>MTMITHHHHHHGSNSYYTEENHGPFELINIGPLPLEEGRCMPECLLAVAVHGALNADKSNAILVPTWYSGTSKAMEQIYIGEGRALDPSKYCIIVVNQIGNGLSSSASNTGGSLAGPGFANVRIGDDVSAQHTLLTEYFGIESLALVVGGSMGAQQTYEWAVRYPDFVKRAAAIAGTARNSEHDFLFTEILIEAITTDPAFQAGLYRSSSAVAAGLERHAKLWTLMGWSPEFFRTGRHK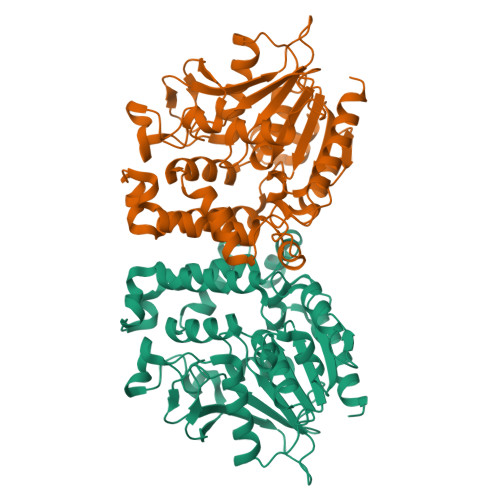ALGFESMQMFVDGFMKRYFAPMDPNNLLTMAWKWQRGDVSRHTGGDLAKALGRIKAKTYVMPISHDQFFTVDDCLSEQKMIPNSEFRPLRSIDGHLGLFGTDAQMLDQLDAHLAELLSSPAY[2x]> MICSGPQNLAQELK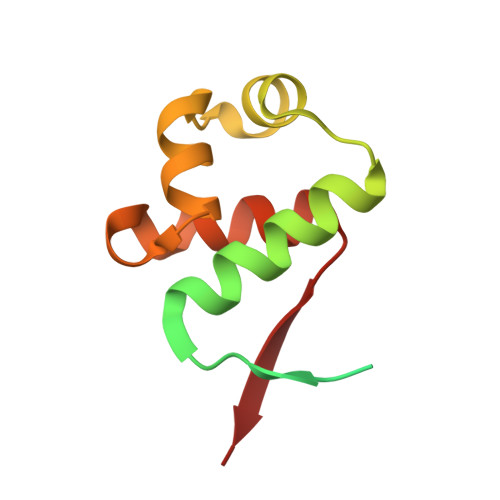AIGDQLQELQKKLIQGPNISQPRPLLTIETPRHLGEQLNARRKELGIDLYTLELQTGISTSTLKRLFKDPEQVKFGSVFAVANVLGVKLCIGE> GSMEELQKSIGHKPEPTDEEWELIKTVTEAHVATNAQGSHWKQKRKFLPEDIGQAPIVNAPEGGKVDLEAFSHFTKIITPAITRVVD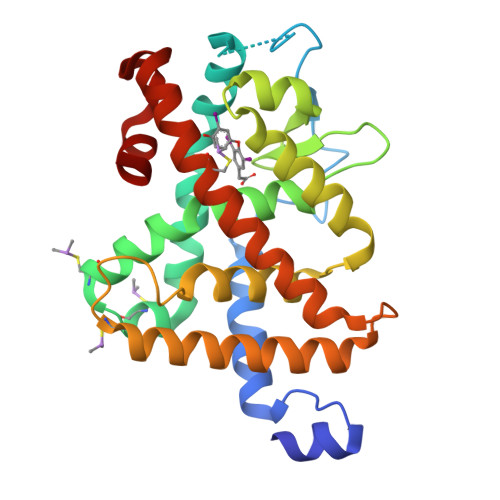FAKKLPMFCELPCEDQIILLKGCCMEIMSLRAAVRYDPESETLTLNGEMAVTRGQLKNGGLGVVSDAIFDLGMSLSSFNLDDTEVALLQAVLLMSSDRPGLACVERIEKYQDSFLLAFEHYINYRKHHVTHFWPKLLMKVTDLRMIGACHASRFLHMKVECPTELFPPLFLEVFED>XEWEALEKKCAALES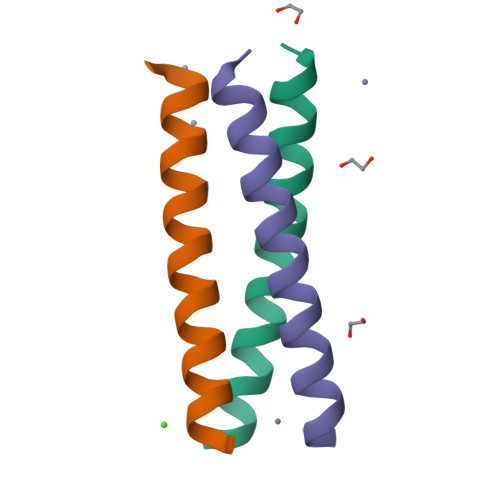KLQALEKKLEALEHGX[3x]> NQPYRTGFHFQPPKNWMNDPNGPMIYKGIYHLFYQWNPKGAVWGNIVWAHSTSTDLINWDPHPPA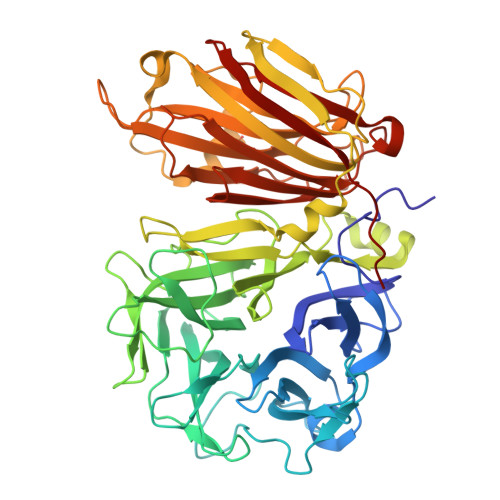IFPSAPFDINGCWSGSATILPNGKPVILYTGIDPKNQQVQNIAEPKNLSDPYLREWKKSPLNPLMAPDAVNGINASSFRDPTTAWLGQDKKWRVIIGSKIHRRGLAITYTSKDFLKWEKSPEPLHYDDGSGMWECPDFFPVTRFGSNGVETSSFGEPNEILKHVLKISLDDTKHDYYTIGTYDRVKDKFVPDNGFKMDGTAPRYDYGKYYASKTFFDSAKNRRILWGWTNESSSVEDDVEKGWSGIQTIPRKIWLDRSGKQLIQWPVREVERLRTKQVKNLRNKVLKSGSRLEVYGVTAAQADVEVLFKVRDLEKADVIEPSWTDPQLICSKMNVSVKSGLGPFGLMVLASKNLEEYTSVYFRIFKARQNSNKYVVLMCSDQSRSSLKEDNDKTTYGAFVDINPHQPLSLRALIDHSVVESFGGKGRACITSRVYPKLAIGKSSHLFAFNYGYQSVDVLNLNAWSMNSAQIS(2R)-N-(4-chlorophenyl)-2-[(1R,3S,5S,6r)-3-(5,6-difluoro-1H-benzimidazol-1-yl)bicyclo[3.1.0]hexan-6-yl]propanamide 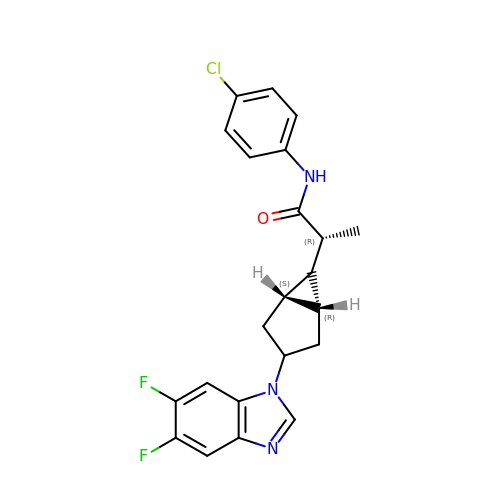| C22 H20 Cl F2 N3 O | FVIXADGZFNVGRM-IDJJVQAESA-N>MSSEQLHEPAELLSEETKNMHRALVTLIEELEAVDWYQQRADACSEPGLHDVLIHNKNEEVEHAMMTLEWIRRRSPVFDAHMRTYLFTERPILELEEEDTGSSSSVAASPTSAPSHGSLGIGSLRQEGKED[5x];>[5x]MDLLKRHLAPIVPDAWSAIDEEAKEIFQGHLAGRKLVDFRGPFGWEYAAVNTGELRPIDDTPEDVDMKLRQVQPLAEVRVPFTLDVTELDSVARGATNPDLDDVARAAERMVEAEDSAIFHGWAQAGIKGIVDSTPHEALAVASVSDFPRAVLSAADTLRKAG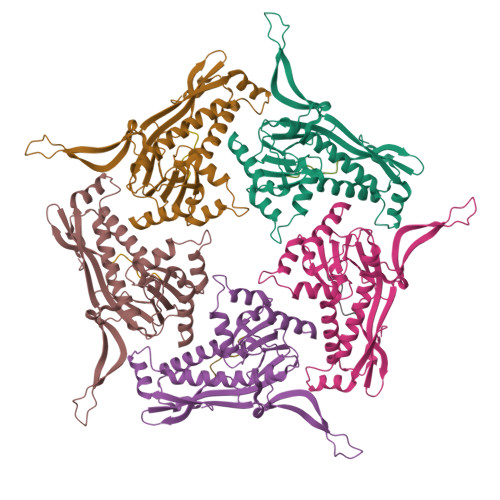VTGPYALVLGPKAYDDLFAATQDGYPVAKQVQRLVVDGPLVRANALAGALVMSMRGGDYELTVGQDLSIGYAFHDRSKVELFVAESFTFRVLEPGAAVHLRYA> GSHMKYHVGIDVGTFSVGLAAIEVDDAGMPIKTLSLVSHIHDSGLDPDEIKSAVTRLASSGIARRTRRLYRRKRRRLQQLDKFIQRQGWPVIELEDYSDPLYPWKVRAELAASYIADEKERGEKLSVALRHIARHRGWRNPYAKVSSLYLPDGPSDAFKAIREEIKRASGQPVPETATVGQMVTLCELGTLKLRGEGGVLSARLQQSDYAREIQEICRMQEIGQELYRKIIDVVFAAESPKGSASSRVGKDPLQPGKNRALKASDAFQRYRIAALIGNLRVRVDGEKRILSVEEKNLVFDHLVNLTPKKEPEWVTIAEILGIDRGQLIGTATMTDDGERAGARPPTHDTNRSIVNSRIAPLVDWWKTASALEQHAMVKALSNAEVDDFDSPEGAKVQAFFADLDDDVHAKLDSLHLPVGRAAYSEDTLVRLTRRMLSDGVDLYTARLQEFGIEPSWTPPTPRIGEPVGNPAVDRVLKTVSRWLESATKTWGAPERVIIEHGGGSGGSMESVAWMANELRSRVAQHFASHGTTVRVYRGSLTAEARRASGISGKLKFFDGVGKSRLDRRHHAIDAAVIAFTSDYVAETLAVRSNLKQSQAHRQEAPQWREFTGKDAEHRAAWRVWCQKMEKLSALLTEDLRDDRVVVMSNVRLRLGNGSAHKETIGKLSKVKLSSQLSVSDIDKASSEALWCALTREPGFDPKEGLPANPERHIRVNGTHVYAGDNIGLFPVSAGSIALRGGYAELGSSFHHARVYKITSGKKPAFAMLRVYTIDLLPYRNQDLFSVELKPQTMSMRQAEKKLRDALATGNAEYLGWLVVDDELVVDTSKIATDQVKAVEAELGTIRRWRVDGFFSPSKLRLRPLQMSKEGIKKESAPELSKIIDRPGWLPAVNKLFSDGNVTVVRRDSLGRVRLESTAHLPVTWKVQ

Besides the crRNA-target DNA complementarity, DNA recognition by Cas9 requires a protospacer adjacent motif (PAM), a specific DNA sequence located downstream of the target sequence. The HNH domain cleaves the DNA strand complementary to the crRNA guide (the target strand), while the RuvC domain cleaves the non-complementary strand (the non-target strand). We confirmed that CdCas9 recognizes the NNRHHHY PAM, and found that CdCas9 efficiently cleaves the double-stranded DNA target, when programmed with the 22-nt guide sgRNA. We thus concluded that, unlike the other Cas9 orthologs, CdCas9 recognizes the promiscuous NNRHHHY PAM, with a preference for adenine at the fourth to sixth PAM nucleotides.

Since we failed to obtain diffraction-quality crystals, we crystallized a CdCas9-∆HNH variant, in which the HNH domain (residues 498–663) is replaced by a GGGSGG linker, as in the case of CjCas99. We determined the crystal structure of CdCas9-∆HNH in complex with a 112-nt sgRNA (a 20-nt guide sequence), a 28-nt target DNA strand, and an 8-nt non-target DNA strand (the GGGTAAT PAM), at 2.9 Å resolution. The crystal structure revealed that CdCas9 adopts a bilobed architecture consisting of the REC and NUC lobes, with the guide RNA-target DNA heteroduplex bound within the central channel, as in the other Cas9 structures. CdCas9-∆HNH comprises five domains, including the RuvC (residues 1–51, 449–497, and 664–807), REC1 (residues 86–235), REC2 (residues 236–448), WED (residues 821–904), and PI (residues 905–1084) domains. In the present structure, the PAM duplex is bound between the WED and PI domains, where the GGGTAAT PAM is recognized by multiple residues in the PI domain. Unexpectedly, the O6 and N7 of dG2* form bidentate hydrogen bonds with Arg1042, despite the lack of an observed preference for the second PAM nucleotide. The N7 of dG3* forms a hydrogen bond with Arg1017, and the R1017A mutant showed almost no activity, confirming the importance of Arg1017 for the PAM recognition. While the nucleobases of dT4*–dA6* in the non-target strand do not form direct contacts with the protein, the nucleobases of dA(−4)–dT(−6) in the target strand are located in the vicinity of a hydrophobic patch formed by Phe1011, Lys1015, Pro1043, and Leu1046. Molecular modeling suggested that the methyl groups of the fourth to sixth T nucleotides in the target strand form van der Waals interactions with the hydrophobic patch, consistent with the preference for the A nucleotides at the fourth to sixth PAM positions. The nucleobase of dT7* does not directly contact the protein, while the N7 of dA(−7) forms a hydrogen bond with Lys1015.>[2x]GSHMKST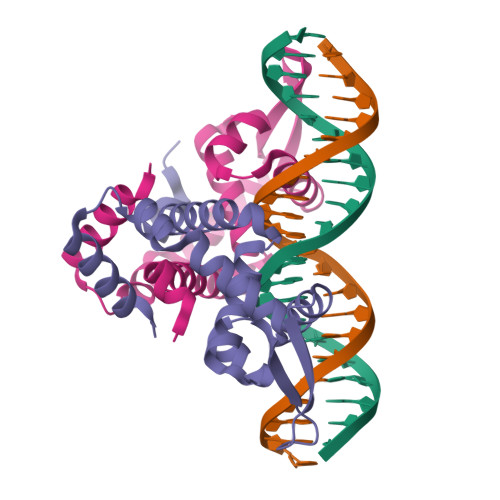SDLFNEIIPLGRLIHMVNQKKDRLLNEYLSPLDITAAQFKVLCSIRCAACITPVELKKVLSVDLGALTRMLDRLVSKGWVERLPNPNDKRGVLVKLTTGGAAICEQCHQLVGQDLHQELTKNLTADEVATLEYLLKKVLP> 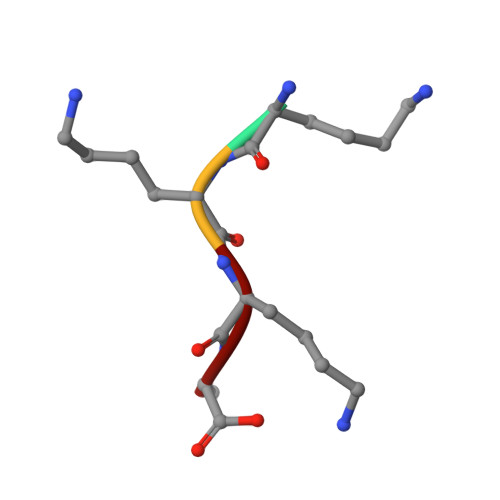KKKA>GMDIINNRRSIRNYKGKKVEKEKIEKLLRAAMQAPSAGNQQPWEFIVLEDRENIDKLSNFSKYANSLKTAPLAIVLLADEEKMKISEMWEQDMAAAAENILLEAAYLDLGAVWLGAQPIEERVKNLKEMFNLKSNIKP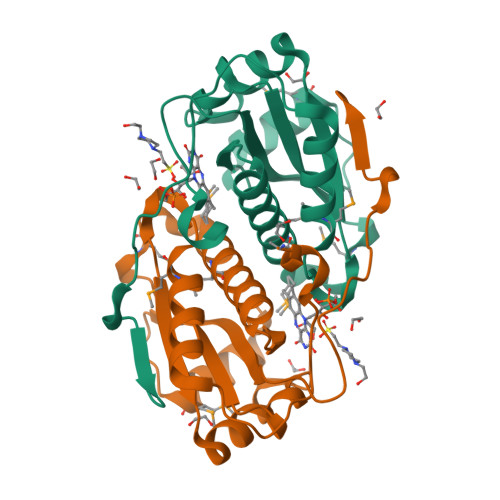FCVISVGYPENSENKFIDRFDAKRIHIEKY[2x]(3S)-3-({[(5S,10aS)-2-{(2S)-4-carboxy-2-[(phenylacetyl)amino]butyl}-1,3-dioxo-2,3,5,7,8,9,10,10a-octahydro-1H-[1,2,4]triazolo[1,2-a]cinnolin-5-yl]carbonyl}amino)-4-oxopentanoic 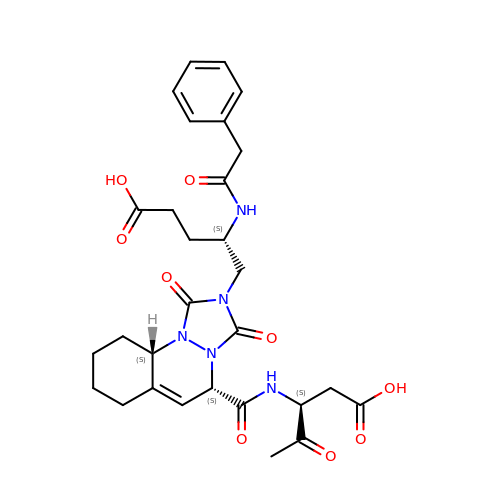acid | C29 H35 N5 O9 | BGEXQSKGWCDSIQ-MLCQCVOFSA-N>GPLGSPSENIQEINTAISDNYTYNIPGIVNNNPFYILFTVNTTGIYKINAQNNLPSLKIYEAIGSGNRNFQSGNLCDDDIKAINYITGFDSPNAKSYLVVLLNKDKNYYIRVPQTSSNIENQIQFKREEGDLRNLMNSSVNIIDNLNSTGAHYYTRQSPDVHDYISYEFTIPGNFNNKDTSNIRLYTSYNQGIGTLFRVTETIDGYNLINIQQNLHLLNNTNSIRLLNGAIYILKVEVTELNNYNIRLHIDITN[2x];>EHYSVIQNSLNDKIVTISCKADTNLFFYQVAGNVSLFQQTRNYLERWRLIYDSNKAAYKIKSMDIHNTNLVLTWNAPTHNISTQQDSNADNQYWLLLKDIGNNSFIIASYKNPNLVLYADTVARNLKLSTLNNSNYIKFIIEDYIISDLNNFTCKISPILDLNKVVQQVDVTNLNVNLYTWDYGRNQKWTIRYNEEKAAYQFFNTILSNGVLTWIFSNGNTVRVSSSNDQNNDAQYWLINPVSDTDETYTITNLRDTTKALDLYGGQTANGTAIQVFNYHGDDNQKWNIRNPPGSA[4x];>GPSVERTFLPNGNYNIKSIFSGSLYLNPVSKSLTFSNESSANNQKWNVEYMAENRCFKISNVAEPNKYLSYDNFGFISLDSLSNRCYWFPIKIAVNTYIMLSLNKVNELDYAWDIYDTNENILSQPLLLLPNFDIYNSNQMFKLEKI[2x]

Here, we report the complete structure of a bimodular ∼760 kDa BoNT/A large progenitor toxin complex (L-PTC), which is composed of BoNT and four non-toxic bacterial proteins. We found that L-PTC/A consists of two structurally and functionally independent sub-complexes, the M-PTC and the HA complex. The HA complex is composed of HA70, HA17, and HA33 in a 3∶3∶6 stoichiometry and adopts an extended three-blade architecture, whereas the M-PTC is situated on top of the HA complex platform. BoNT/A absorption is mainly mediated by nine glycan-binding sites on the HA complex that together form multivalent interactions with host carbohydrate receptors on intestinal epithelial cells.

We next separated the HA complex into two major components: the central hub composed of homo-trimeric HA70 and the blade composed of HA70D3–HA17–HA33. Their crystal structures were determined at 2.9 Å and 3.7 Å, respectively. Specifically, homo-trimeric HA70 forms the core of the complex with each C-terminal HA70D3 domain binding to one HA17, which in turn simultaneously coordinates two HA33s. Each HA adopts an almost identical conformation in the independently solved structures, despite differences in crystal packing, suggesting that they represent physiologically relevant conformations. The 12-subunit HA complex is stabilized by numerous protein–protein interactions that include interactions among the HA70s of the central trimer, between HA70 and HA17, between HA17 and the two HA33 molecules, and between the two HA33s in each blade. The N-terminal domain of HA33 is fixed in the HA complex through extensive inter-HA33 and HA17–HA33 interactions, but its C-terminal domain is largely unrestricted.>[2x]MNTQLMGERIRARRKKLKIRQAALGKMVGVSNVAISQWERSETEPNGENLLAL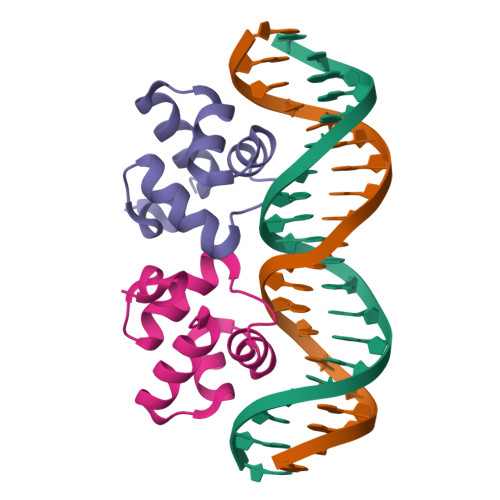SKALQCSPDYLLKGD2-({5-CHLORO-2-[(2-METHOXY-4-MORPHOLIN-4-YLPHENYL)AMINO]PYRIMIDIN-4-YL}AMINO)-N-METHYLBENZAMIDE | C23 H25 Cl N6 O3 | 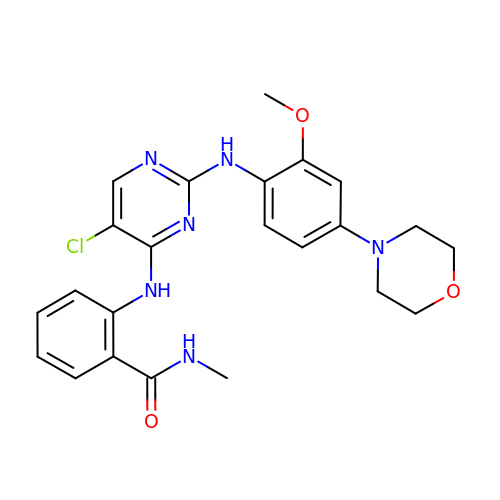UYJNQQDJUOUFQJ-UHFFFAOYSA-N N-(3-AMINOPROPYL)-N-[(R)-(3-BENZYL-5-CHLORO-4-OXO-3,4-DIHYDROPYRROLO[2,1-F][1,2,4]TRIAZIN-2-YL)(CYCLOPROPYL)METHYL]-4-METHYLBENZAMIDE 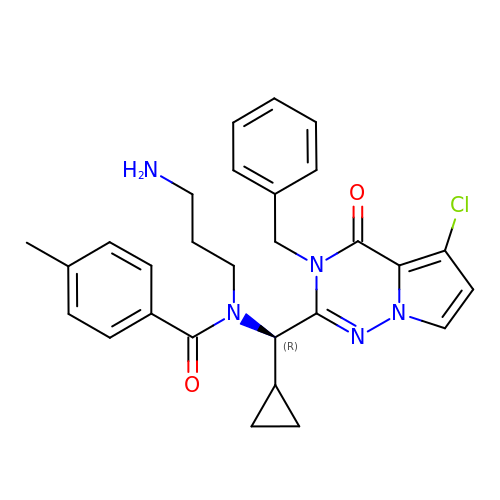| C28 H30 Cl N5 O2 | IKORZPHBTIOSSU-XMMPIXPASA-N>[4x]MWFGEFGGQYVPETLIEPLKELEKAYKRFKDDEEFNRQLNYYLKTWAGRPTPLYYAKRLTEKIGGAKIYLKREDLVHGGAHKTNNAIGQALLAKFMGKTRLIAETGAGQHGVATAMAGALLGMKVDIYMGAEDVERQKMNVFRMKLLGANVIPVNSGSRTLKDAINEALRDWVATFEYTHYLIGSVVGPHPYPTIVRDFQSVIGREAKAQILEAEGQLPDVIVACVGGGSNAMGIFYPFVNDKKVKLVG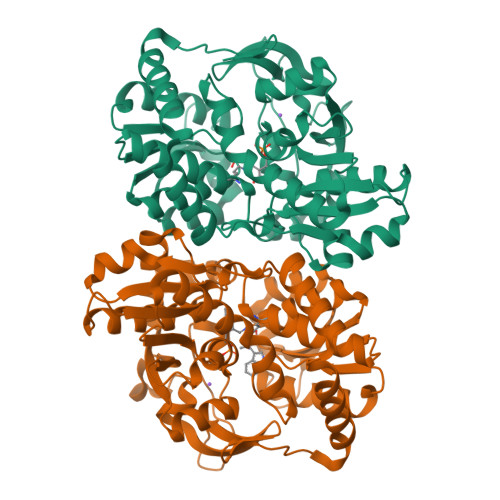VEAGGKGLESGKHSASLNAGQVGVFHGMLSYFLQDEEGQIKPTHSIAPGLDYPGVGPEHAYLKKIQRAEYVTVTDEEALKAFHELSRTEGIIPALESAHAVAYAMKLAKEMSRDEIIIVNLSGRGDKDLDIVLKVSGNVLEHHHHHH Recently, mutational screening analysis identified the chloroplast-localized HJ resolvase MOC1 that is essential for chloroplast nucleoid segregation in Chlamydomonas reinhardtii and Arabidopsis thaliana. MOC1 exhibits dimerization and an RNaseH fold, belonging to the retroviral integrase superfamily. Moreover, we characterize a base recognition loop (BR loop) that protrudes into the junction and disrupts the C–G base pairs at the crossover. Residue D183 from the BR loop recognizes the cytosine, determining the cytosine-dependent HJ resolution.

After tedious trials, we finally determined two crystal structures of the NtMOC1-HJ complex at an approximately 2.5 Å resolution in the P21212 space group. One of the structures contains the active NtMOC1 and HJ with a noncognate CATG core sequence, and the other is composed of a cleavage-inactive NtMOC1 mutant (D116A/E175A/D253A/E258A) and an HJ with a cognate CCGG core sequence. The HJs in both structures are four-stranded with a 9-bp arm length in each direction with only variation in the crossover with either the CATG core or the CCGG core. These two NtMOC1-HJ complexes exhibit a nearly identical overall fold. In the HJs of both complexes, the CATG and CCGG at the branch point were well aligned. Four acidic amino acids, namely D116, D118, E175, and E258, coordinate a magnesium ion approach to the cleavable phosphodiester backbone, constituting the catalytic tetrad. Alanine substitutions of D116, D118, E175 and E258 completely abolished HJ cleavage activity, although the HJ binding activity was retained. Once the cognate sequence of CCGG (or CGCG) moves to the branch point, residues Y180 and D183 from the dynamic BR loop of NtMOC1 could penetrate into the junction and disrupt the C–G base pairs. Meanwhile, the disrupted cytosine is recognized by D183, generating a favorable HJ configuration, thus facilitating the hydrolysis of the phosphodiester bond by the catalytic tetrad of NtMOC1.

>[2x]AHMNAGWVIGVAPDTSGALALLKPNQPPQVFDSPHLKVLVGKGVRKRLDAKAIVQLLKSFEAPIGTTVYVAQSTPYPQDGKQGWWSGGFGYGMWIGILVASGFSVIPVPSSAWKSEFQLTKERSNKDYSRQVASQLFPSLSSLLKRKKAHGRAAALLIAAYGKGIKINS>[2x]PISPIETVPVKLKPGMDGPKVKQWPLTEEKIKALVEICTEMEKEGKISKIGPENPYNTPVFAIKKKDSTKWRKLVDFRELNKRTQDFWEVQLGIPHPAGLKKKKSVTVLDVGDAYFSVPLDEDFRKYTAFTIPSINNETPGIRYQYNVLPQGWKGSPAIFQSSMTKILEPFRKQNPDIVIYQYMDDLYVGSDLEIGQHRTKIEELRQHLLRWGLT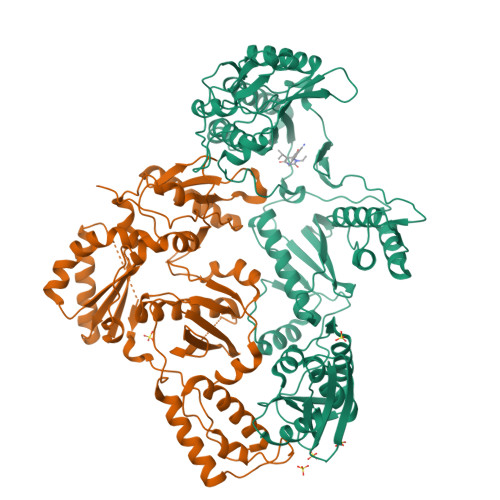TPDKKHQKEPPFLWMGYELHPDKWTVQPIVLPEKDSWTVNDIQKLVGKLNWASQIYPGIKVRQLCKLLRGTKALTEVIPLTEEAELELAENREILKEPVHGVYYDPSKDLIAEIQKQGQGQWTYQIYQEPFKNLKTGKYARMRGAHTNDVKQLTEAVQKITTESIVIWGKTPKFKLPIQKETWETWWTEYWQATWIPEWEFVNTPPLVKLWYQLEKEPIVGAETFYVDGAANRETKLGKAGYVTNRGRQKVVTLTDTTNQKTELQAIYLALQDSGLEVNIVTDSQYALGIIQAQPDQSESELVNQIIEQLIKKEKVYLAWVPAHKGIGGNEQVDKLVSAGIRKVL>[8x]GHMSTLLINQPQYAWLKELGLREENEGVYNGSWGGRGEVITTYCPANNEPIARVRQASVA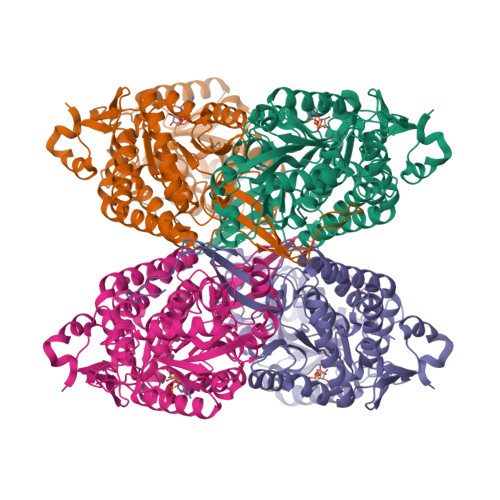DYEETVKKAREAWKIWADIPAPKRGEIVRQIGDALREKIQVLGSLVSLEMGKILVEGVGEVQEYVDICDYAVGLSRMIGGPILPSERSGHALIEQWNPVGLVGIITAFNFPVAVYGWNNAIAMICGNVCLWKGAPTTSLISVAVTKIIAKVLEDNKLPGAICSLTCGGADIGTAMAKDERVNLLSFTGSTQVGKQVGLMVQERFGRSLLELGGNNAIIAFEDADLSLVVPSALFAAVGTAGQRCTTARRLFIHESIHDEVVNRLKKAYAQIRVGNPWDPNVLYGPLHTKQAVSMFLGAVEEAKKEGGTVVYGGKVMDRPGNYVEPTIVTGLGHDASIAHTGTFAPILYVFKFKNEEEVFAWNNEVKQGLSSSIFTKDLGRIFRWLGPKGSDCGIVNVNIPTSGAEIGGAFGGEKHTGGGRESGSDAWKQYMRRSTCTINYSKDLPLAQGIKFQ> SRAFQPEFVESISNVSVAVGRDATFTCHVRHLGGYRVGWLKADTKAIQAIHENVITHNPRVTVSHLDQNTWNLHIKAVSEEDRGGYMCQLNTDPMKSQIGFLDVVIPPDFISEDTSSDVIVPEGSSVRLTCRARGYPEPIVTWRREDGNEIVLKDNVGTKTLAPSFRGEVLKLSKISRNEMGSYLCIASNGVPPSVSKR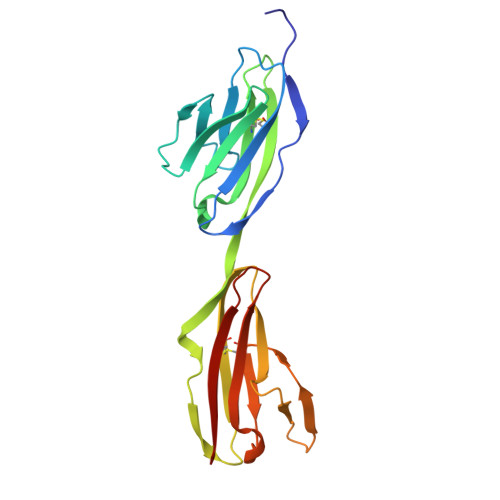ISLSIHH> MGMRGSHHHHHHRPECVVPEFQCAVKRKEKKAQKDKDKPNSTT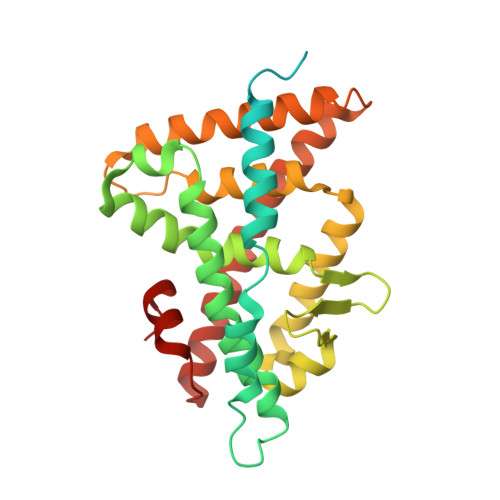SCSPDGIKQEIDPQRLDTDSQLLSVNGVKPITPEQEELIHRLVYFQNEYEHPSPEDIKRIVNAAPEEENVAEERFRHITEITILTVQLIVEFSKRLPGFDKLIREDQIALLKACSSEVMMFRMARRYDAETDSILFATNQPYTRESYTVAGMGDTVEDLLRFCRHMCAMKVDNAEYALLTAIVIFSERPSLSEGWKVEKIQEIYIEALKAYVENRRKPYATTIFAKLLSVLTELRTLGNMNSETCFSLKLKNRKVPSFLEEIWDVVS>[4x]GSH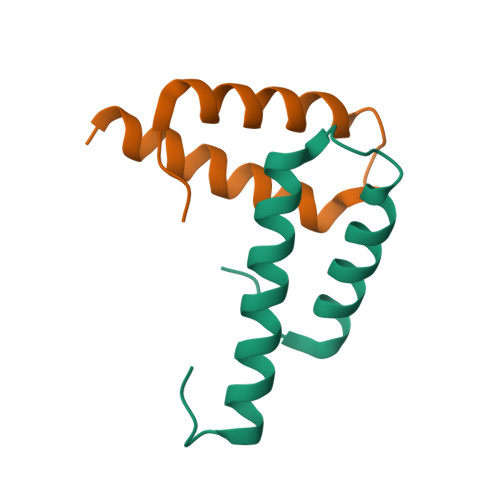EATVEYLADLVKEKKHLTLFPHMFSAVERLLDDEIGRVRVALFQTEFPRVELPEPAG(4-fluoranyl-3-oxidanyl-phenyl)-(6-methylquinolin-2-yl)methanone 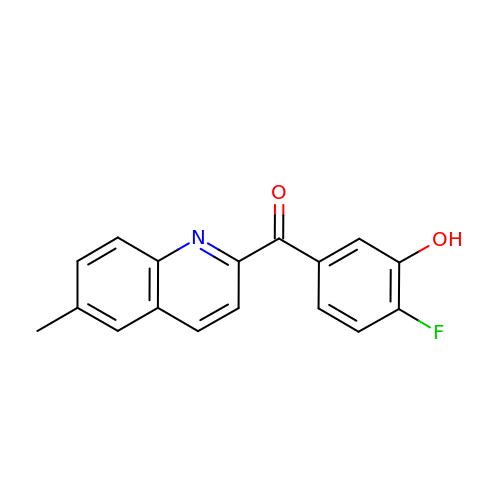| C17 H12 F N O2 | DIBIPWTWYDLKIZ-UHFFFAOYSA-N>GSQIPASE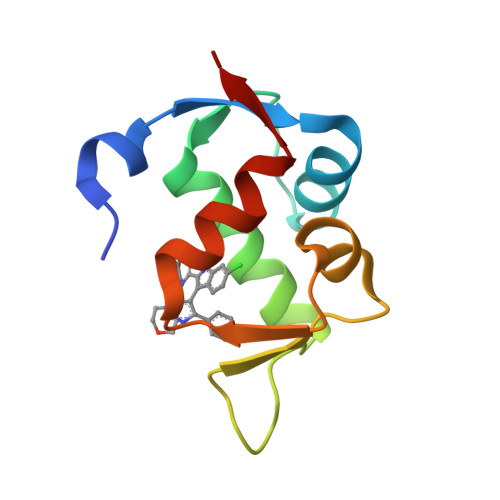QETLVRPKPELLKLLKSVGAQKDTYTMKEVLFYLGQYIMTKRLYDEKQQHIVYCSNDLLGDLFGVPSFSVKEHRKIYTMIYRNLVVVN[2x]>MMSNRSDFIVPDEAAVKRAASVNFHLEPLRPWLDDPQITEVCVNRPGEVFCERASAWEYYAVPNLDYEHLISLGTATARFVDQDISDSRPVLSAILPMGERIQIVRPPACEHGTISVTIRKPSFTRRTLEDYAQQGFFKHVRPMSKSLTPFEQELLALKEAGDYMSFLRRAVQLERVIVVAGETGSGKTTLMKALMQEIPFDQRLITIEDVPELFLPDHPNHVHLFYPSEAKEEENAPVTAATLLRSCLRMKPTRILLAELRGGEAYDFINVAASGHGGSITSCHAGSCE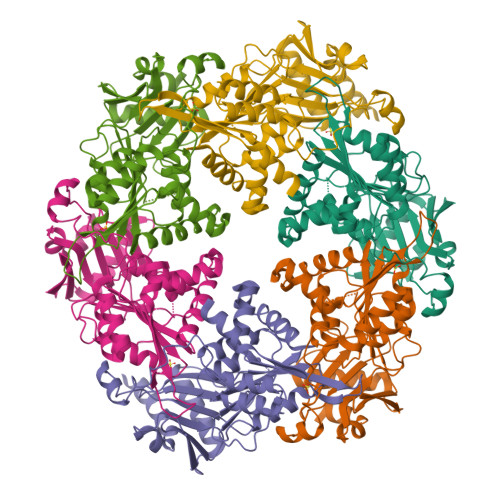LTFERLALMVLQNRQGRQLPYEIIRRLLYLVVDVVVHVHNGVHDGTGRHISEVWYDPNTKRALSLQHSEKT[3x]> MEGFKANLSLLRRPGEKTYTQRCRLFVGNLPADITEDEFKRLFAKYGEPGEVFINKGKGFGFIKLESRALAEIAKAELDDTPMRGRQLRVRFATHAAALSVRNLSPYVSNELLEEAFSQFGPIERAVVIVDDRGRSTGKGIVEFASKPAARKAFERCSEGVFLLTTTPRPVIVEPLEQLDDEDGLPEKLAQKNPMYQKERETPPRFAQHGTFEYEYSQRWKSLDEMEKQQREQVEKNMKDAKDKLESEMEDAYHEHQANLL;> GMGFTIDIKSFLKPGEKTYTQRCRLFVGNLPTDITEEDFKRLFERY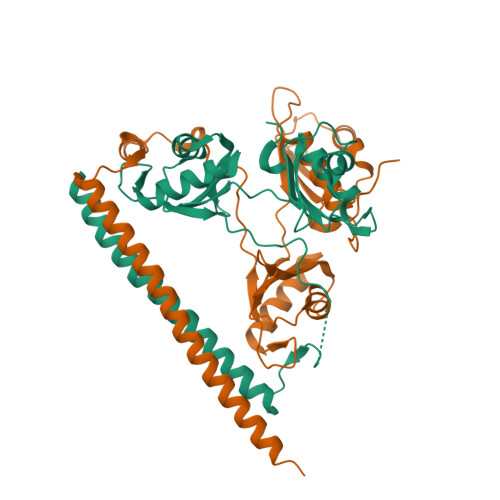GEPSEVFINRDRGFGFIRLESRTLAEIAKAELDGTILKSRPLRIRFATHGAALTVKNLSPVVSNELLEQAFSQFGPVEKAVVVVDDRGRATGKGFVEFAAKPPARKALERCGDGAFLLTTTPRPVIVEPMEQFDDEDGLPEKLMQKTQQYHKEREQPPRFAQPGTFEFEYASRWKALDEMEKQQREQVDRNIREAKEKLEAEMEAARHEHQLMLM> GSPGISGGGGGSQNSLALHKVIMVGSGGVGKSALTLQFMYDEFVEDYEPTKADSYRKKVVLDGEEVQIDILDTAGQEDYAAIRDNYFRSGEGFLCVFSITEMESFAATADFREQILRVKEDENVPFLLVGNKSDLEDKRQVSVEEAKNRAEQWNVNYVETSAKTRANVDKVFF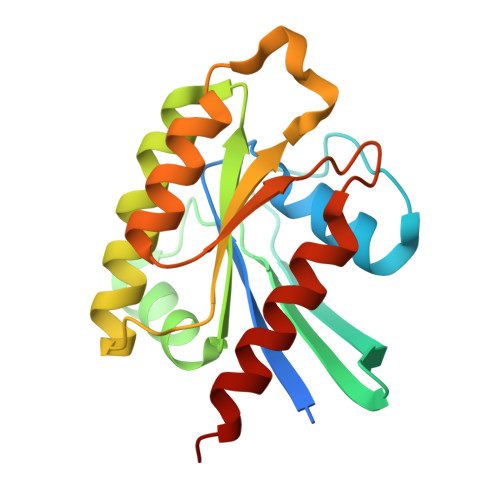DLMREIRARKMEDS N-(2-amino-1H-benzimidazol-5-yl)-2-[3-[(2-amino-2-oxoethyl)-methylsulfonylamino]-5-chlorophenyl]acetamide 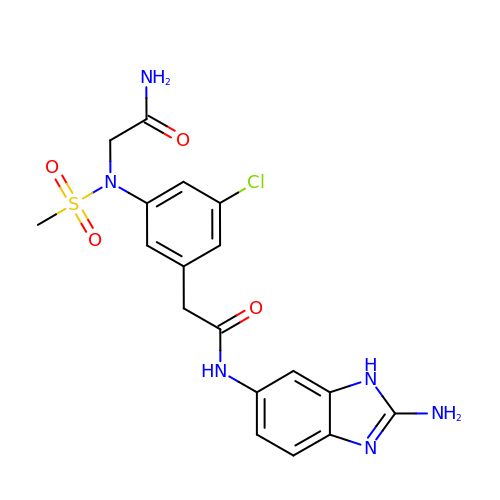| C18 H19 Cl N6 O4 S | YEZPHSBANAZNOO-UHFFFAOYSA-N> MKRNYILGLDIGITSVGYGIIDYETRDVIDAGVRLFKEANVENNEGRRSKRGARRLKRRRRHRIQRVKKLLFDYNLLTDHSELSGINPYEARVKGLSQKLSEEEFSAALLHLAKRRGVHNVNEVEEDTGNELSTKEQISRNSKALEEKYVAELQLERLKKDGEVRGSINRFKTSDYVKEAKQLLKVQKAYHQLDQSFIDTYIDLLETRRTYYEGPGEGSPFGWKDIKEWYEMLMGHCTYFPEELRSVKYAYNADLYNALNDLNNLVITRDENEKLEYYEKFQIIENVFKQKKKPTLKQIAKEILVNEEDIKGYRVTSTGKPEFTNLKVYHDIKDITARKEIIENAELLDQIAKILTIYQSSEDIQEELTNLNSELTQEEIEQISNLKGYTGTHNLSLKAINLILDELWHTNDNQIAIFNRLKLVPKKVDLSQQKEIPTTLVDDFILSPVVKRSFIQSIKVINAIIKKYGLPNDIIIELAREKNSKDAQKMINEMQKRNRQTNERIEEIIRTTGKENAKYLIEKIKLHDMQEGKCLYSLEAIPLEDLLNNPFNYEVDHIIPRSVSF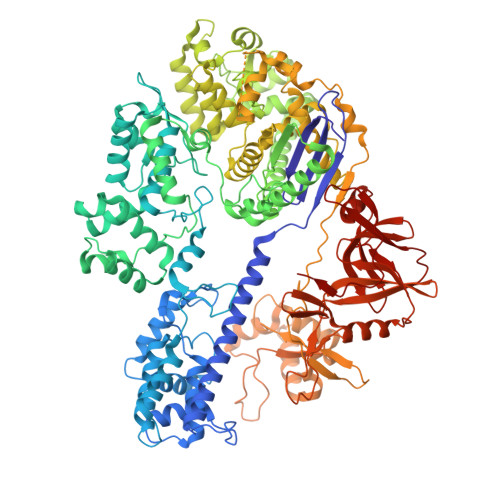DNSFNNKVLVKQEENSKKGNRTPFQYLSSSDSKISYETFKKHILNLAKGKGRISKTKKEYLLEERDINRFSVQKDFINRNLVDTRYATRGLMNLLRSYFRVNNLDVKVKSINGGFTSFLRRKWKFKKERNKGYKHHAEDALIIANADFIFKEWKKLDKAKKVMENQMFEEKQAESMPEIETEQEYKEIFITPHQIKHIKDFKDYKYSHRVDKKPNRELINDTLYSTRKDDKGNTLIVNNLNGLYDKDNDKLKKLINKSPEKLLMYHHDPQTYQKLKLIMEQYGDEKNPLYKYYEETGNYLTKYSKKDNGPVIKKIKYYGNKLNAHLDITDDYPNSRNKVVKLSLKPYRFDVYLDNGVYKFVTVKNLDVIKKENYYEVNSKCYEEAKKLKKISNQAEFIASFYNNDLIKINGELYRVIGVNNDLLNRIEVNMIDITYREYLENMNDKRPPRIIKTIASKTQSIKKYSTDILGNLYEVKSKKHPQIIKKG> MDSFWFVQQWPPAVCSFQKSGSCPGSGLRTFTIHGLWPQQSGTS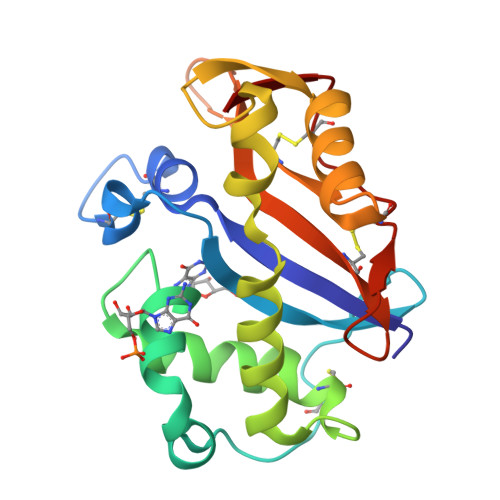LTNCPGSPFDITKISHLQSQLNTLWPSVLRANNQQFWSHEWTKHGTCSESTFNQAAYFKLAVDMRNNYDIIGALRPHAAGPNGRTKSRQAIKGFLKAKFGKFPGLRCRTDPQTKVSYLVEVVACFAQDGSTLIDCTRDTCGANFIF>[2x]GSMVTVEEVRKAQRAEGPATVLAIGTATPSNCVDQATYPDYYFRITNSEHKTELKEKFQRMCDKSMIKKRYMYLTEEILKENPTVCEYMAPSLDARQDMVVVEVPRLGKEAATKAIKEWGQPKSKITHLVFCTTSGVDMPGADYQLTKLLGLRPYVKRLMMYQQGCFAGGTVLRLAKDLAENNKGARVLVVCSEITAVTFRGPSDTHLDSLVGQALFGDGAAAVIIGADPLPEVEKPLFELVSAA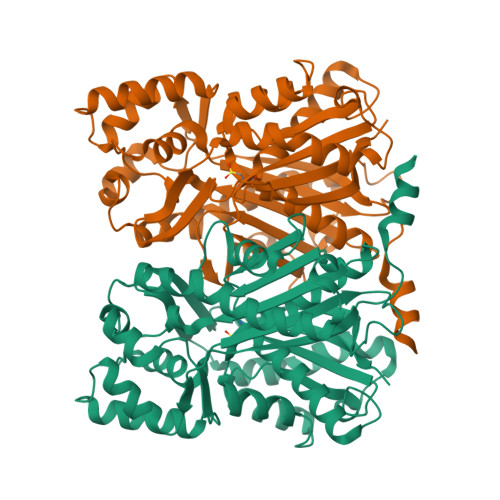QTILPDSDGAIDGHLREVGLTFHLLKDVPGLISKNIEKSLNEAFKPIGISDWNSLFWIAHPGGPAILDQVESKLALKPEKLEATRQVLSNYGNMSSACVLFILDEVRRKSTEKGLRTTGEGLEWGVLFGFGPGLTVETVVLHSVA> GHMASNVANDGERPSRVVE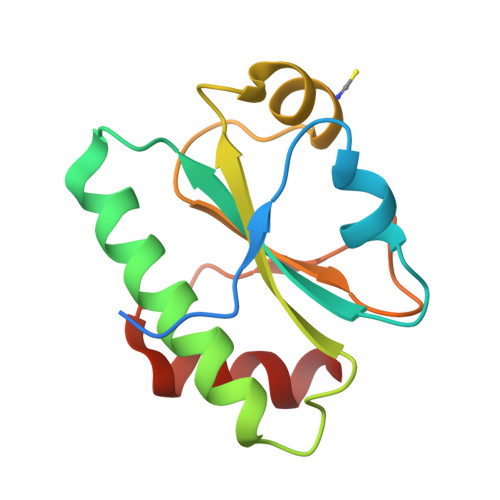LTDETFDSIVMDPEKDVFVLYYVPWSRHSVAAMRLWDDLSMSQSQKRNHLTFVAARIDGEKYPDVIERMRVSGFPTMRYYTRIDKQEPFEYSGQRYLSLVDSFVFQNT>[2x]MSGAPPGYRPSAWVHLLHQLPRADFQLRPVPSVFAPQEQEYQQALLLVAALAGLGLGLSLIFIAVYLIRFCCCRPPEPPGSKIPSPGGGCVTWSCIVALLAGCTGIGIGFYGNSETSDGVSQLSSALLHANHTLSTIDHLVLETVERLGEAVRTELTTLEEVLEPRTELVAAARGARRQAEAAAQQLQGLAFWQGVPLSPLQVAENVSFVEEYRWLAYVLLLLLELLVCLFTLLGLAKQSKWLVIVMTVMSLLVLVLSWGSMGLEAATAVGLSDFCSNPDPYVLNLTQEETGLSSDILSYYLLCNRAVSNPFQQRLTLSQRALANIHSQLLGLEREAVPQFPSAQKPLLSLEETLNVTEGNFHQLVALLHCRSLHKDYGAALRGLCEDALEGLLFLLLFSLLSAGALATALCSLPRAWALFPPSDDYDDTDDDDPFNPQESKRFVQWQSSIALEVLFQ

The Tweety homologs (TTYHs) are members of a conserved family of eukaryotic membrane proteins that are abundant in the brain. The three human paralogs were assigned to function as anion channels that are either activated by Ca2+ or cell swelling. All TTYH molecules are dimers and contain an extended extracellular domain, five membrane spanning segments, and an unstructured cytoplasmic region. In light of its distinct protein architecture and the absence of functional evidence for ion transport, we thus conclude that the TTYH family does not form ion channels and instead confers other catalytic properties.

To obtain a comprehensive overview of TTYH conformations, we have investigated the structural properties of all three paralogs in distinct environments: The structures of TTYH2 and 1 were determined in GDN under Ca2+-free conditions at 3.3 and 4.0 Å, respectively. Both proteins display a novel fold with very similar general features. Whereas in both structures of TTYH2 determined in detergent and in lipid nanodiscs, the two transmembrane domains (TMDs) are separated by about 7 Å and thus not in direct contact, they have approached each other in the TTYH1 and 3 structures by mutual rigid body rotations of subunits by 6–7° around an axis located at the extracellular dimer interface. The described conformational differences lead to interactions in the transmembrane parts of TTYH1 and 3, which increase the contact area between interacting subunits to 2600 and 3655 Å2, respectively. In contrast to contacts in the extracellular domain, the interactions between subunits within the membrane region observed for TTYH1 and 3 are hydrophobic. Additionally, there are contacts between the TMDs of TTYH1 and 3 but not of TTYH2. On a subunit level, all three paralogs are generally similar, which is reflected in the low root-mean-square deviation of 2.3 and 2.5 Å calculated from superpositions of Cα atoms of TTYH2 with TTYH1 and 3, respectively. While residual density is also found in the data of TTYH1, its detailed distribution differs owing to the distinct shape of the cavity at its extracellular end.>GSHMELTEDLN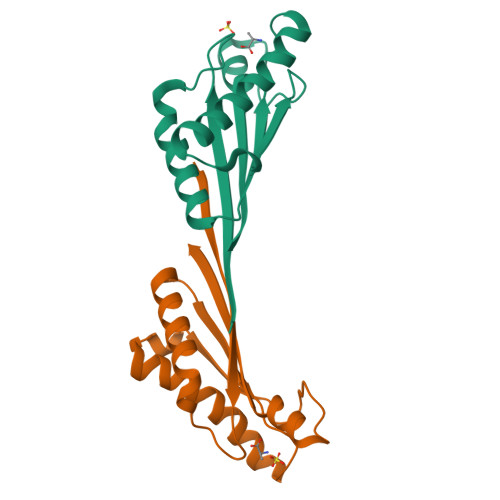MELRVFFDTNKSNIKDQYKPEIAKVAEKLSEYPNATARIEGHTDNTGPRKLNERLSLARANSVKSALVNEYNVDASRLSTQGFAWDQPIADNKTKEGRAMNRRVFATITGSR[8x]> SNALEDAQESKALVNMPGPSSESLGKDDKPISLQNWKRGLDILSPMERFHLKYLYVTDLATQNWCELQTAYGK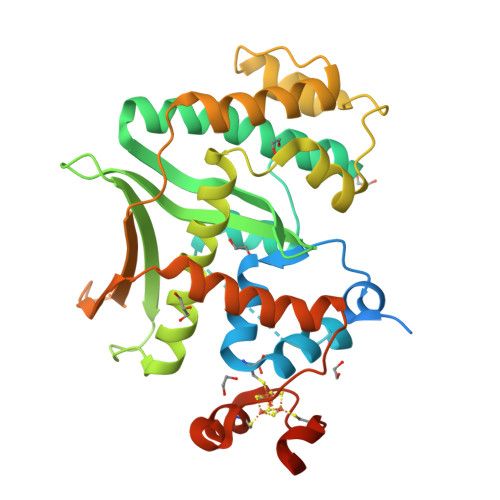ELPGFLAPEKAAVLDTGASIHLARELELHDLVTVPVTTKEDAWAIKFLNILLLIPTLQSEGHIREFPVFGEVEGVLLVGVIDELHYTAKGELELAELKTRRRPMLPLEAQKKKDCFQVSLYKYIFDAMVQGKVTPASLIHHTKLCLEKPLGPSVLRHAQQGGFSVKSLGDLMELVFLSLTLSDLPVIDILKIEYIHQETATVLGTEIVAFKEKEVRAKVQHYMAYWMGHREPQGVDVEEAWKCRTCTYADICEWRKGSGVLSSTLAPQVKKAK3-[(2R)-2-ethylpiperidin-1-yl]-N-[6-({3-[(2S)-2-ethylpiperidin-1-yl]propanoyl}amino)acridin-3-yl]propanamide 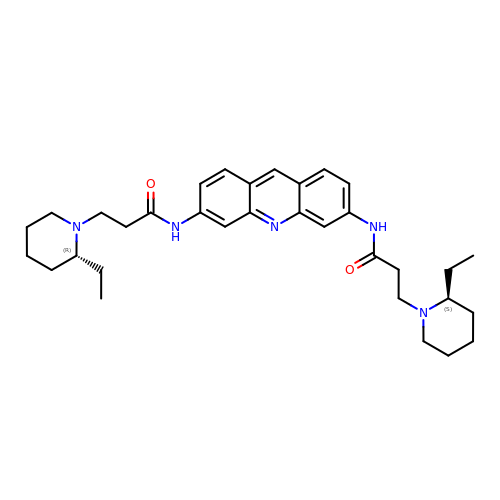| C33 H45 N5 O2 | ZWPUGYBFVBXUSX-ISILISOKSA-N{3-[(1R)-3-(3,4-dimethoxyphenyl)-1-({[(2S)-1-{[(1S,2R)-2-ethyl-1-hydroxycyclohexyl](oxo)acetyl}piperidin-2-yl]carbonyl}oxy)propyl]phenoxy}acetic acid | C35 H45 N O10 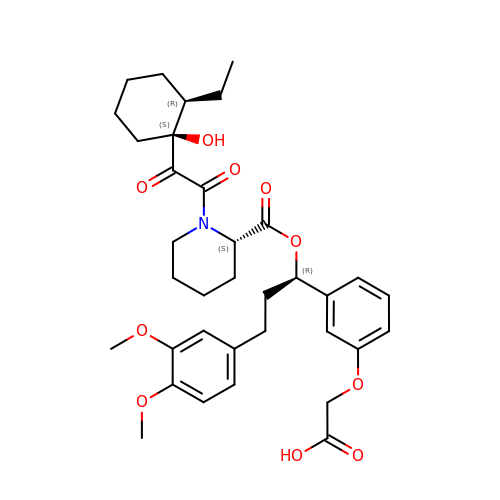| JLRDMSUQFUWACS-XACWCOMZSA-N1-(3-{5-[(3-chlorobenzyl)sulfonyl]-1H-tetrazol-1-yl}phenyl)ethanone | C16 H13 Cl N4 O3 S | 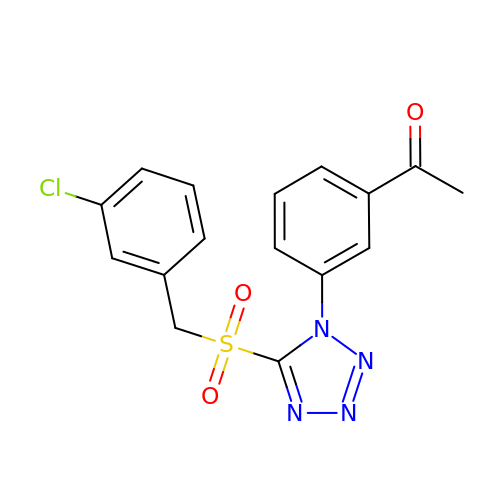VMFCIDSTIJTUES-UHFFFAOYSA-N>[2x]MSRSKRDNNFYSVEIGDSTFTVLKRYQNLKPIGSGAQGIVCAAYDAILERNVAIKKLSRPFQNQTHAKRAYRELVLMKCVN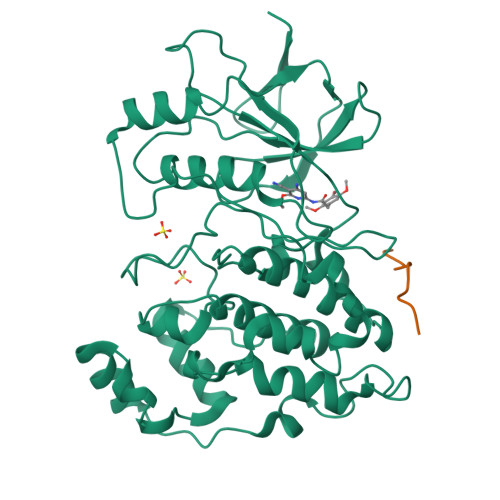HKNIIGLLNVFTPQKSLEEFQDVYIVMELMDANLCQVIQMELDHERMSYLLYQMLCGIKHLHSAGIIHRDLKPSNIVVKSDCTLKILDFGLARTAGTSFMMEPEVVTRYYRAPEVILGMGYKENVDLWSVGCIMGEMVCHKILFPGRDYIDQWNKVIEQLGTPCPEFMKKLQPTVRTYVENRPKYAGYSFEKLFPDVLFPADSEHNKLKASQARDLLSKMLVIDASKRISVDEALQHPYINVWYDPSEAEAPPPKIPDKQLDEREHTIEEWKELIYKEVMDLEHHHHHH;>[2x]RPKRPTTLNLF>[2x]TTRDRVPTYQYNMNFEKLGKCIIINNKNFDKVTGMGVRNGTDKDAEALFKCFRSLGFDVIVYNDCSCAKMQDLLKKASEEDHTNAACFACILLSHGEENVIYGKDGVTPIKDLTAHFRGARCKTLLEKPKLFFIQACRGTELDDGIQADSGPINDTDANPRYKIPVEADFLFAYSTVPGYYSWRSPGRGSWFVQALCSILEEHGKDLEIMQILTRVNDR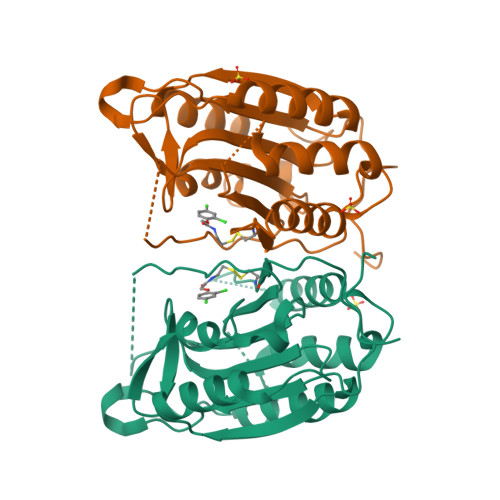VARHFESQSDDPHFHEKKQIPCVVSMLTKELYFSQQLHHHHHH>[2x]HHHHHHVSASPLKVAVTGAAGQIGYSLLFRLASGSLLGPDRPIELRLLEIEPALQALEGVVMELDDCAFPLLSGVEIGSDPQKIFDGVSLALLVGARPRGAGMERSDLLEA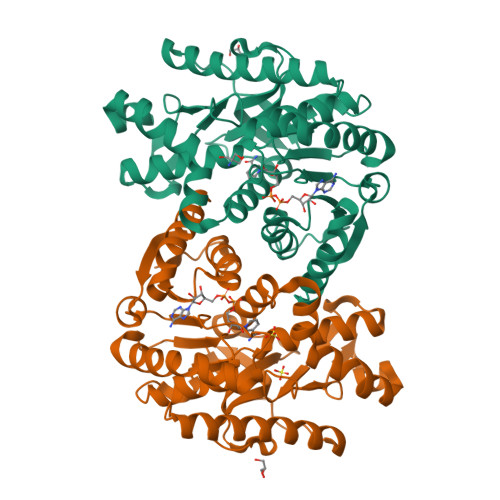NGAIFTAQGKALNAVAADDVRVGVTGNPANTNALIAMTNAPDIPRERFSALTRLDHNRAISQLAAKTGAAVTDIKKMTIWGNHSATQYPDLFHAEVAGKNAAEVVNDQAWIEDEFIPTVAKRGAAIIDARGASSAASAASATIDAARDWLLGTPADDWVSMAVVSDGSYGVPEGLISSFPVTTKGGNWTIVSGLEIDEFSRGRIDKSTAELADERSAVTELGLI>[5x]GPGSMSLSTAVSGGG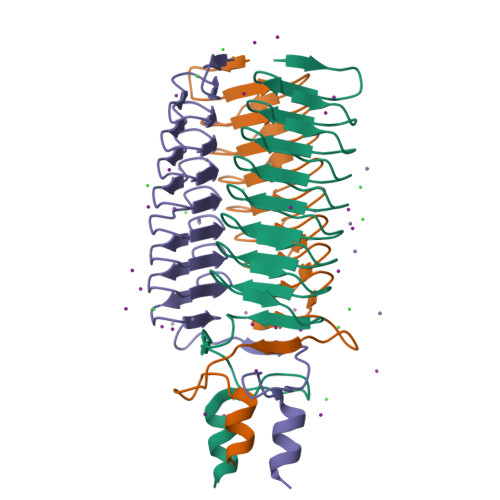VRTSSLGDTSAGNGANASGGNGTAVGGAASASGTDATALGQASNASGNHSTALGQASSASGSGSTAVGQGAGAPGDGASAFGQGALASGTDSTALGAHSTAAAPNSAAIGANSVASAPNSVSFGSRGHERRLTNVAPGIDGTDAANMNQLWGVQSSVDQAARR> MAPWKIEEVKTLKGLIKSKPVVAIVDMMDVPAPQLQEIRDKIRDKVKLR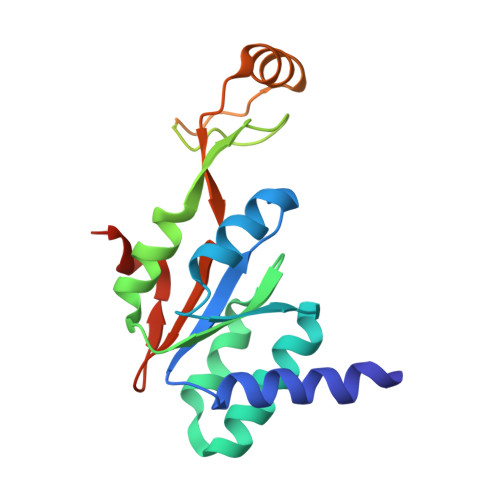MSRNTLIIRALKEAAEELNNPKLAELANYVERGAAILVTDMNPFKLYKLLEENKSPAPVRGGQIAPCDIKVEKGSTGMPPGPFLGELKSVGIPAAIEKGKIAIKEDKVVVKKGEVVSPKLAAVLDRLGIKPIKVGLNILAVYEDGIIYTPDVLKVDEEKLLADI>[4x]MAHHHHHHMTDESSVRTPKALPDGVSQATVGVRGGMLRSGFEETAEAMYLTSGYVYGSAAVAEKSFAGELDHYVYSRYGNPTVSVFEERLRLIEGAPAAFATASGMAAVFTSLGALLGAGDRLVAARSLFGSCFVVCSEILPRWGVQTVFVDGDDLSQWERA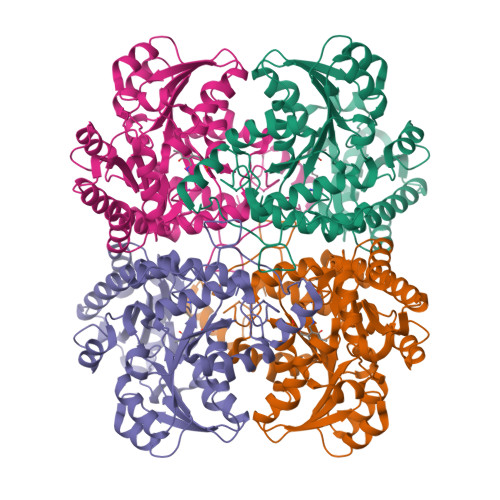LSVPTQAVFFETPSNPMQSLVDIAAVTELAHAAGAKVVLDNVFATPLLQQGFPLGVDVVVYSGTKHIDGQGRVLGGAILGDREYIDGPVQKLMRHTGPAMSAFNAWVLLKGLETLAIRVQHSNASAQRIAEFLNGHPSVRWVRYPYLPSHPQYDLAKRQMSGGGTVVTFALDCPEDVAKQRAFEVLDKMRLIDISNNLGDAKSLVTHPATTTHRAMGPEGRAAIGLGDGVVRISVGLEDTDDLIADIDRALS>HF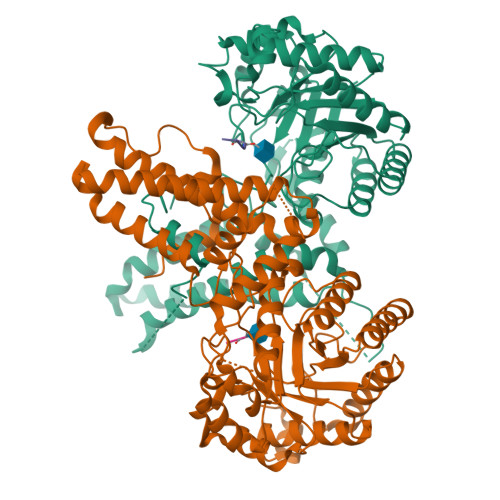LCGVVEGFYGRPWVMEQRKELFRRLQKWELNTYLYAPKDDYKHRMFWREMYSVEEAEQLMTLISAAREYEIEFIYAISPGLDITFSNPKEVSTLKRKLDQVSQFGCRSFALLFDNIDHNMCAADKEVFSSFAHAQVSITNEIYQYLGEPETFLFCPTEYCGTFCYPNVSQSPYLRTVGEKLLPGIEVLWTGPKVVSKEIPVESIEEVSKIIKRAPVIWDNIHANDYDQKRLFLGPYKGRSTELIPRLKGVLTNPNCEFEANYVAIHTLATWYKSNMNGVRKDVVMTDSEDSTVSIQIKLENEGSDEDIETDVLYSPQMALKLALTEWLQEFGVPHQYSSRGGGGSGGGGSVTLEDLQLLADLFYLPYEHGPKGAQMLREFQWLRANSSVVSVNCKGKDSEKIEEWRSRAAKFEEMCGLVMGMFTRLSNCANRTILYDMYSYVWDIKSIMSMVKSFVQWLGCRSHSSAQFLIGDQEPWAFRGGLAGEFQRLLPIDGANDLFFQ[2x];>[2x]VPYSSAQ> MSQEALKAPVVVLGAGLASVSFVAELRQAGYQGLITVVGDEAERPYDRPPLSKDFMAHGDAEKIRLDCKRAPEVEWLLGVTAQSFDPQAHTVALSDGRTLPYGTLVLATGAAPRALPTLQGATMPVHTLRTLEDARRIQAGLRPQSRLLIVGGGVIGLELAATARTAGVHVSLVCRGPRLMSRAAPATLADFVARYHAAQGVDLRFERSVTGSVDGVVLLDDGTRIAADMVVVGIGVLANDALARAAGLACDDGIFVDAYGRTTCPDVYALGDVTRQRNPLSGRFERIETWSNAQNQGIAVARHLVDPTAPGYAELPW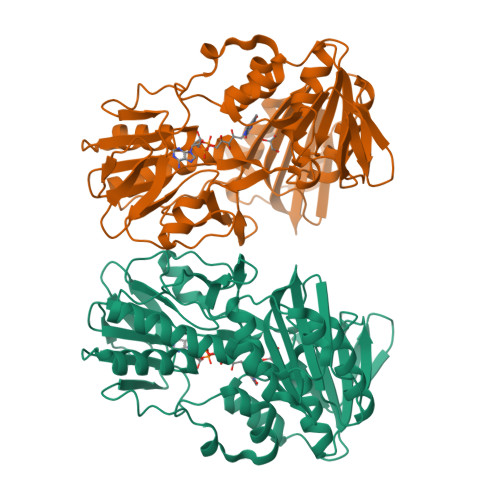YWSDQGALRIQVAGLASGDEEIVRGEVSLDAPKFTLIELQKGRIVGATCVNNARDFAPLRRLLAVGAKPDRAALADPATDLRKLAAAVAA> SYYST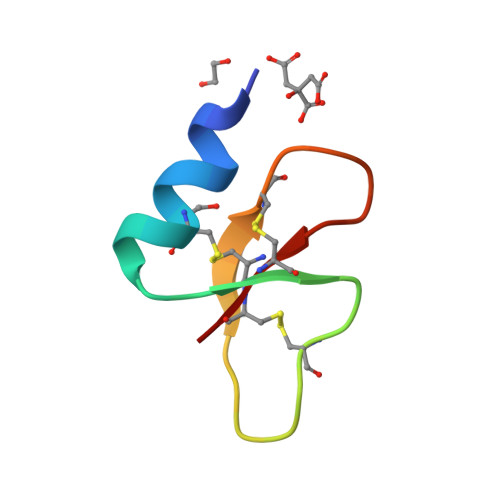LQCRNNHGHCRRLCFHGEQWIGNCNGRHQHCCK>[2x]MTNKISSSDNLSNAVSATDDNASRTPNLNRRALVGGGVGLAARGALASGLQAATLPAGASQVPTTPAGRPMPYAIRPMPEDRRFGYAIVGLGKYALNQILPGFAGCQHSRIEALVSGNAEKAKIVAAEYGVDPRKIYDYSNFDKIAKDPKIDAVYIILPNSLHAEFAI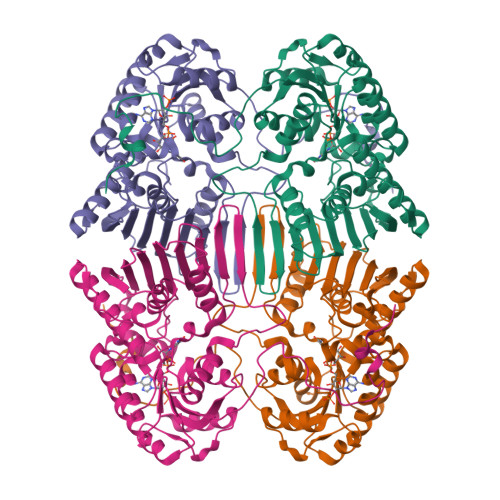RAFKAGKHVMCEKPMATSVADCQRMIDAAKAANKKLMIGYRCHYDPMNRAAVKLIRENQLGKLGMVTTDNSDVMDQNDPAQQWRLRRELAGGGSLMDIGIYGLNGTRYLLGEEPIEVRAYTYSDPNDERFVEVEDRIIWQMRFRSGALSHGASSYSTTTTSRFSVQGDKAVLLMDPATGYYQNLISVQTPGHANQSMMPQFIMPANNQFSAQLDHLAEAVINNKPVRSPGEEGMQDVRLIQAIYEAARTGRPVNTDWGYVRQGGY>MNDSSVIYRAIVTSKFRTEKMLNFYNSIGSGPDKNTIFITFG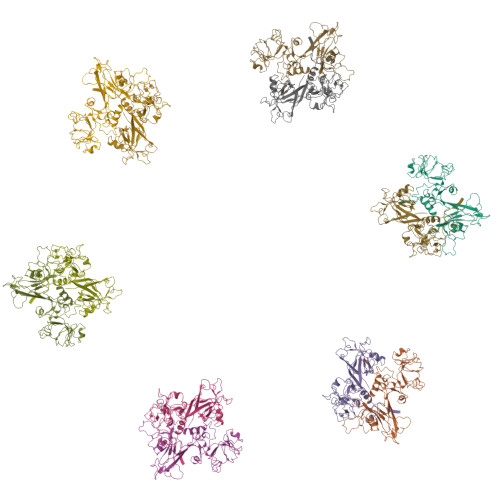RSEPWSSNENEVGFAPPYPTDSVLGVTDMWTHMMGTVKVLPSMLDAVIPRRDWGDTRYPDPYTFRINDIVVCNSAPYNATESGAGWLVYRCLDVPDTGMCSIASLTDKDECLKLGGKWTPSARSMTPPEGRGDAEGTIEPGDGYVWEYLFEIPPDVSINRCTNEYIVVPWPEELKEDPTRWGYEDNLTWQQDDFGLIYRVKANTIRFKAYLDSVYFPEAALPGNKGFRQISIITNPLEAKAHPNDPNVKAEKDYYDPEDLMRHSGEMIYMENRPPIIMAMDQTEEINILFTF[12x]> MSTQLASNIYAPLYAPFFGFAGCAAAMVLSCLGAAIGTAKSGIGIAGIGTFKPELIMKSLIPVVMSGIL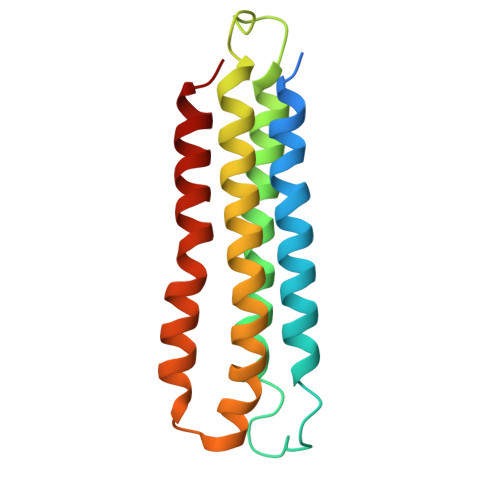AIYGLVVAVLIAGNLSPTEDYTLFNGFMHLSCGLCVGFACLSSGYAIGMVGDVGVRKYMHQPRLFVGIVLILIFSEVLGLYGMIVALILNTRGSE>TKPGYINAAFRSSKNNEAYFFINDKYVLLDYAPGSSRDKVLYGPTPVRDGFKSLNQTIFGSYGIDCSFDTENNEAFIFYENFCALI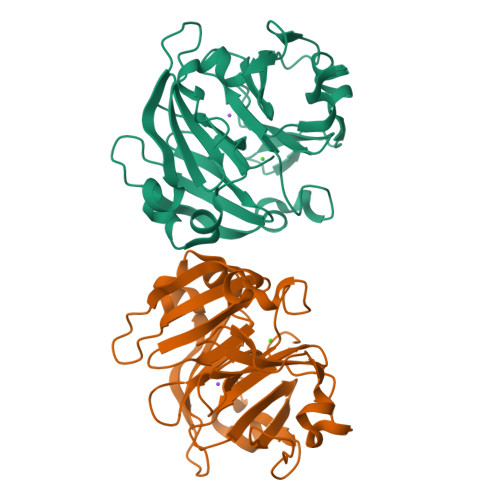DYAPHSKKDKIILGPKKIADVFPFFEGTVFESGIDAAYRSTRGKEVYLFKGDQYARIDYGSNSMVNKEIKSISSGYPCFRNTIFESGADAAFASHKTNEVYFFKDDHYARVKVTPXXKLXIMDGVREIVDYWPSLKDIVPL[4x]5-CHLORO-THIOPHENE-2-CARBOXYLIC ACID ((3R,5S)-1-{[2-FLUORO-4-(2-OXO-PYRIDIN-1-YL)-PHENYLCARBAMOYL]-METHYL}-5-HYDROXYMETHYL-PYRROLIDIN-3-YL)-AMIDE | C23 H22 Cl F 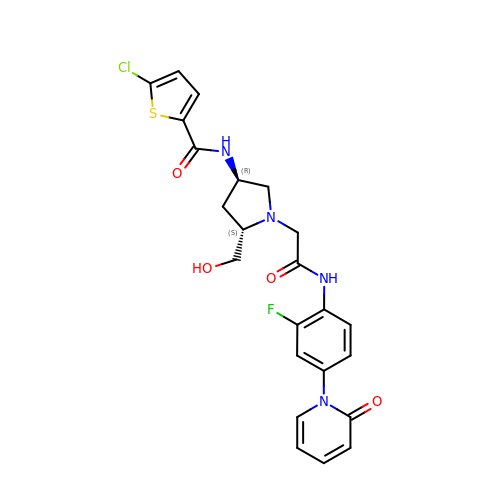N4 O4 S | FMLMGXAAZAZCMG-ZBFHGGJFSA-N>GPLGSMSPPPAESHIILLIQQGSDPKTRIWSDHCSLRSAIEYIVGVYQTNQAVSEKESIDVSRFFNFFDEIYDCVPLVYDRHFRAYIP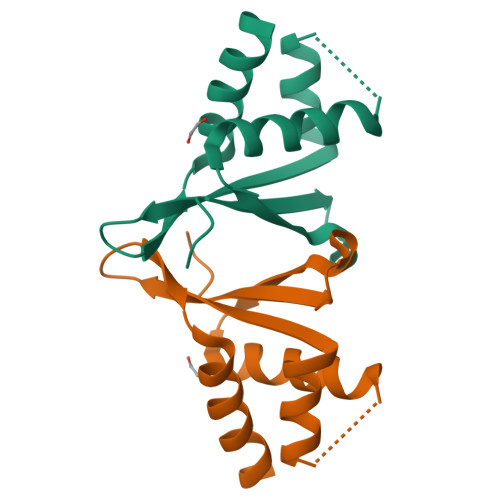HEKQWLLHHAQEYLTAARQIP[3x]> MDINDKLSIDSPIDNKNIIEFITFRTDTSGIQKKIKAYQIAKHIWVVPERYYAEPLNISDEYKIDGGIYNENYLTTDKERQEYLDAICILFKRINNVIEGKKLLSLLSSASPFPFKDDTNKYLLKEALLYVNEENFEFKFFTSNIILFGPGTNISKNQVLPLNGDDATSGVGSVSEICYNPFFTKKFGEYSLDPVIGLIECLLKSLYNLYGIKVSDDIKIPYKLQRALNTDKYSYINLEEALIFGGNDYKIFTEKPYWLSN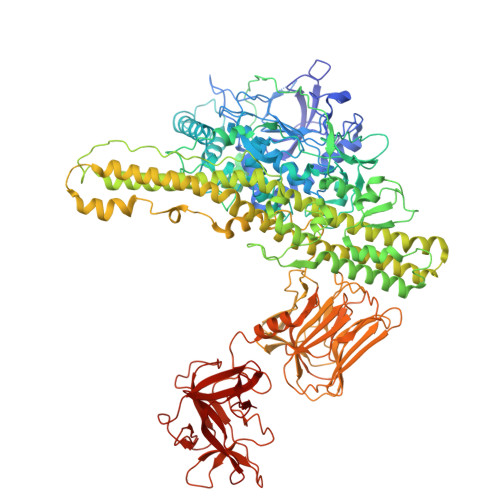DYFLKSLNTFEENKAKYEKDLKNDPNLNNELNQYLQQKYSFSISKIWSLNLTAFADIFNINIPTSFLASITFWDRSQYYKINYPNDYNIDGFVNGQWNTNLKNIEKDNNFIIFDKPKQIITYINDIFNLRYTSNLYEDNLDIESNNYYLNFMFEYDKGNNFTINQYKALLDTLDNDFIDSLPPIQGMNAQNKLTSLPIISKGTDTENINSELLLPIHYLKSQTYNLDMYSSIKFTTNIYEVVSEKNSELVYTFLPHINEIMENYSINNTIKTEEEFYNWMENLFINYSIDILEKRNSIIPGITAVLPWIGKALNILNTNNDFEEELQLSGIKGLIKEYENFIIPDMIVPDIPLDNMPRTYDDIDKKLSEIYTKNKFLFLKGYYFIVQEWWTTYYIQFIELKYLCSGAINKQQQLLITVLEKQLFYFTNNGLFPFDAMERMINEFNRSIDIFSRISQQALNNVDIFINECALFIFNNEVYPLFLNNVENNINKANDNVLNYINKATSLTEEQIKELTVKYTFSSIAEVEFFNESYFKKITNMDIKNILTNIKNINNLILSGSQINDDITIFDESGNNLNIKFDPSIRIVDGHTNVAFKLDKSSQYINIPTENINFSFMESFSIDFWLKILDSTESTTLLNCIEDDIGWKLSIQNNNLLWEMKDNLGNNFTSLFTFNINNIWHNITLSIDRLTNTFNCFLDGKLINTDNISNIFSLETNTPIEIQSDNGAILLEAFSILNYPLQQQEVLNRYREAFSNNYTRNYYGDILKYNENYQLYNKTSPDKEVKKVFTNDKDYIAIEYNQNTNNPTFFSLIQKEQSKIYVEENDEVYICVQGDPLNYITIDNNQAVLTKDINLATSFKLKTNLNKPNSLIFSENSQALRLSNRLNDENYILLDLVSKLDDEPLNIFYWEFI5-amino-3-(methylsulfanyl)-1H-pyrazole-1,4-dicarboxamide | C6 H9 N5 O2 S | 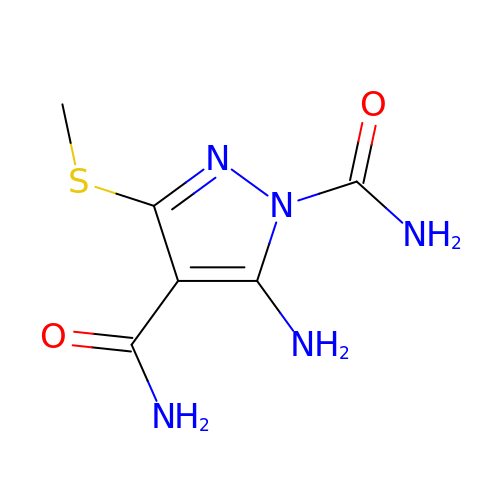TUVCBRIDRHWVLF-UHFFFAOYSA-N The two gel-forming mucins MUC5AC and MUC5B constitute the main structural components of the mucus protecting the underlying epithelia in the respiratory system. The VWD assemblies are formed by the VWD domain, C8, trypsin inhibitor like (TIL) and E domains, except the VWD’ domain that only has the TIL and E domains. We determined the cryoEM structures of the wild type D3 assembly of the human MUC5AC mucin and the structural single nucleotide polymorphisms (SNP) variants Arg996Gln and Arg1201Trp that affect intermolecular interactions. The D3 assembly forms covalent dimers that can appear in two alternative conformations, open and closed, where the closed conformation dimers interact through an arginine-rich loop in the TIL3 domain to form tetramers.

We produced recombinant proteins with each variant separate as well as with both arginines replaced. The general appearance of the dimers is essentially identical. In the double mutant, the effect of the Arg996Gln mutation is more pronounced, bringing the VWD3 and the TIL3 domain closest together. The double mutant shows that once Arg996 is mutated, Trp1201 stabilizes the interface bringing TIL3 closer to VWD3. The double mutant Arg996Gln Arg1201Trp showed a ratio of 96:4 confirming the effect of the mutations. Even though no major rearrangements were found, both SNPs can affect the equilibrium between the dimer open and closed conformation. A high prevalence of double mutants is not observed except in Finnish population, where both mutants are present independently in 10.9% and 23.9%.

>[2x]DAAQPARRAVRSSRHHHHHHGSATCAVYGDGHYLTFDGQSYSFNGDCEYTLVQNHCGGKDSTQDSFRVVTENVPCGTTGTTCSKAIKIFLGGFELKLSHGKVEVIGTDESQEVPYTIQQMGIYLVVDTDIGLVLLWDKKTSIFINLSPEFKGRVCGLCGNFDDIAVNDFATRSRSVVGDVLEFGNSWKLSPSCPDALAPKDPCTANPFRKSWAQKQCSILHGPTFAACHAHVEPARYYEACVNDACACDSGGDCECFCTAVAAYAQACHEVGLCVSWRTPSICPLFCDYYNPEGQCEWHYQPCGVPCLRTCRNPRGDCLRDVWGLEGCYPKCPPEAPIFDEDKMQCVATCPTPPLPPRCHVHGKSYRPGAVVPSDKNCQSCLCTERGVECTYKAEACVCTYNGQRFHPGDVIYHTTDGTGGCISARCGANGTIERRVYPCSPTTPVPPTTFSFSTPPLVVSSTHTPSNGPSSAHTGPPSSAWPTTAGTDDDDKTSEQKLISEEDLSRKLTR> EVIERNHVLILGWSDKLGSLLKQLAIANKSVGGGVIVVLAEKEKEEMEMDIAKLEFDFMGTSVICRSGSPLILADLKKVSVSKARAIIVLAADENADQSDARALRVVLSLAGVKEGLRGHVVVEMSDLDNEPLVKLVGGELIETVVAHDVIGRLMIQCALQPGLAQIWEDILGFENAE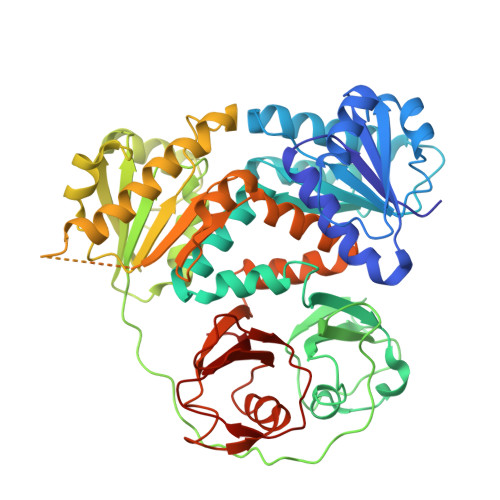FYIKRWPELDDLLFKDILISFPDAIPCGVKVAADGGKIVINPDDNYVLRDGDEVLVIAEDDDTYAPGPLPEVRKGYFPRIRDPPKYPEKILFCGWRRDIDDMIMVLEAFLAPGSELWMFNEVPEKERERKLAAGELDVFGLENIKLVHREGNAVIRRHLESLPLETFDSILILADESVEDSVAHSDSRSLATLLLIRDIQSRRLPYRDTKSTSLRLSGFSHNSWIREMQQASDKSIIISEILDSRTRNLVSVSRISDYVLSNELVSMALAMVAEDKQINRVLEELFAEEGNEMCIKPAEFYLFDQEELCFYDIMIRGRTRKEIVIGYRLANQERAIINPSEKSVPRKWSLDDVFVVLASG> AECSVDIQGNDQMQFNTNAITVDKSCKQFTVNLSHPGNLP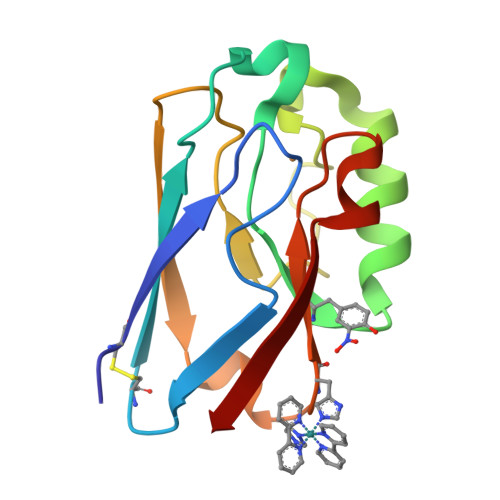KNVMGHNFVLSTAADMQGVVTDGMASGLDKDFLKPDDSRVIAHTKLIGSGEKDSVTFDVSKLKEEEHFYFFCTFPGHSALMKGTLTLK>MAPVKVFGPAMSTNVARVTLCLEEVGAEYEVVDIDFKAMEHKSPEHLVRNPFGQIPAFQDGDLLLFESRAIAKYVLRKYKTDEVDLLREGNLKEAAMVDVWTEVDAHTYNPALSPIVYECLINPLMRGLPTNQTVVDESLEKLKKVLEVYEARLSQHKYLAGDFVSFADLNHFPYTFYFMATPHAALFDSYPHVKAWWDRLM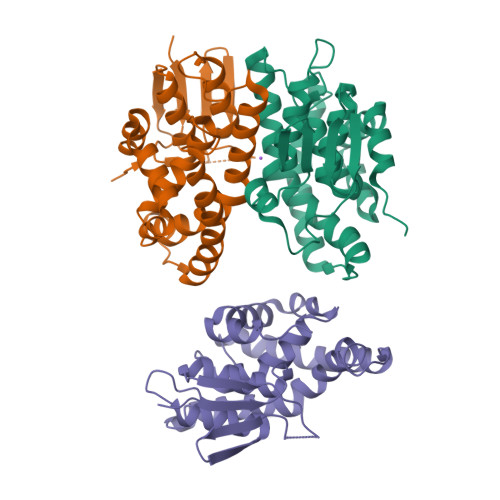ARPAVKKIAATMVPPKAHHHHHH[3x]CYTIDINE 5'-MONOPHOSPHATE 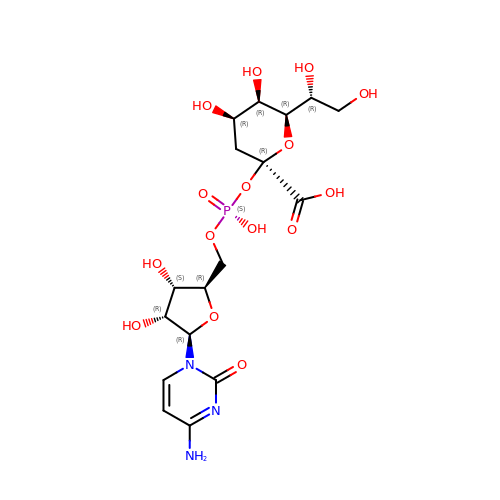3-DEOXY-BETA-D-GULO-OCT-2-ULO-PYRANOSONIC ACID | C17 H26 N3 O15 P | YWWJKULNWGRYAS-UOVSKDHASA-N> GLGDELEEVIVEKTKQTVASISSGPKHTQKVPILTANETGATMPVLPSDSIETRTTYMHFNGSETDVECFLGRAACVHVTEIQNKDA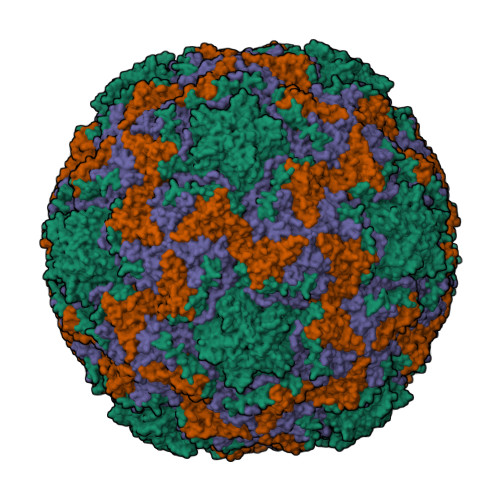TGIDNHREAKLFNDWKISLSSLVQLRKKLELFTYVRFDSEYTILATASQPDSANYSSNLVVQAMYVPPGAPNPKEWDDYTWQSASNPSVFFKVGDTSRFSVPYVGLASAYNCFYDGYSHDDAETQYGITVLNHMGSMAFRIVNEHDEHKTLVKIRVYHRAKHVEAWIPRAPRALPYTSIGRTNYPKNTEPVIKKRKGDIKSY;> SPNVEACGYSDRVQQITLGNSTITTQEAANAVVCYAEWPEYLPDVDASDVNKTSKPDTSVCRFYTLDSKTWTTGSKGWCWKLPDALKDMGVFGQNMFFHSLGRSGYTVHVQCNATKFHSGCLLVVVIPEHQLASHEGGNVSVKYTFTHPGERGIDLSSANEVGGPVKDVLYNMNGTLLGNLLIFPHQFINLRTNNTATIVIPYINSVPIDSMTRHNNVSLMVIPIAPLTVPTGATPSLPITVTIAPMCTEFSGIRSKSIVPQ;> GLPTTTLPGSGQFLTTDDRQSPSALPNYEPTPRIHIPGKVHNLLEIIQVDTLIPMNNTHTKDEVNSYLIPLNANRQNEQVFGTNLFIGDGVFKTTLLGEIVQYYTHWSGSLRFSLMYTGPALSSAKLILAYTPPGARGPQDRREAMLGTHVVWDIGLQSTIVMTIPWTSGVQFRYTDPDTYTSAGFLSCWYQTSLILPPETTGQVYLLSFISACPDFKLRLMKDTQTISQTVALTE;> GAQVSTQKSGSHENQNILTNGSNQTFTVINYYKDAASTSSAGQSLSMDPSKFTEPVKDLMLKGAPALN> GSAEEWYFGKITRRESERLLLNPENPRGTFLVRESETTKGAYCLSVSDFDNAKGLNVKH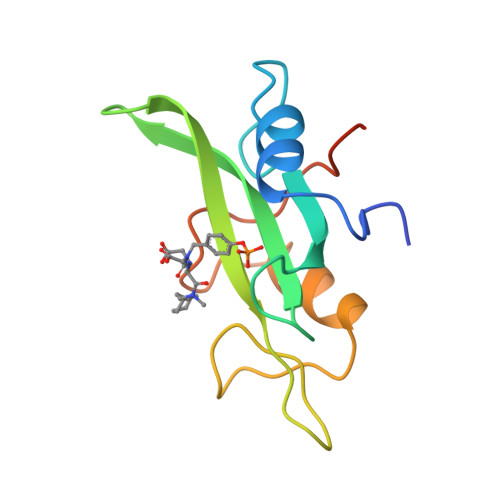YKIRKLDSGGFYITSRTQFSSLQQLVAYYSKHADGLCHRLTNVCPTSKEFIVTD>GPLGSGGLFFNALKNCKENFTVLQTIRQQQSTLNGSWVALLQTRNTLNRAGIRYMMDQNNIGSGSTVAELMESASISLKQAEKNWADYEALPRDPRQSTAAAAEIKRNYDIYHNALAELIQLLGAGKINEFFDQPTQGYQDGFEKQ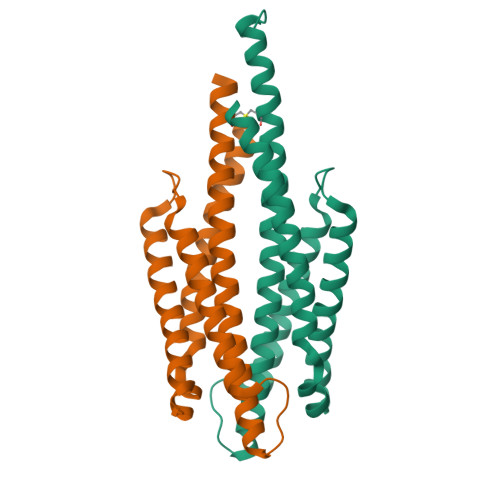YVAYMEQNDRLHDIAVSDNNASYSHHHHHH[2x]> IVGGTASVRGEWPWQVTLHTTSPTQRHLCGGSIIGNQWILTAAHCFYGVESPKILR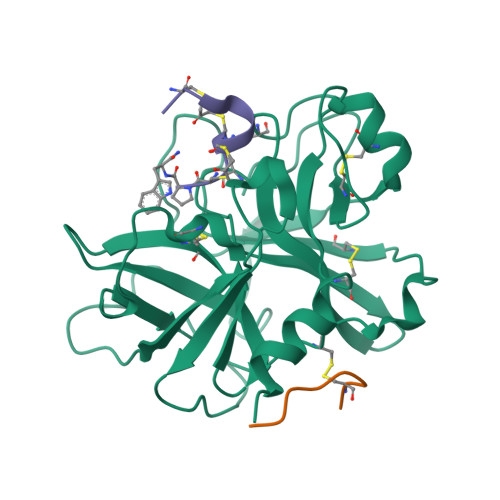VYSGILNQSEIKEDTSFFGVQEIIIHDQYKMAESGYDIALLKLETTVGYGDSQRPICLPSKGDRNVIYTDCWVTGWGYRKLRDKIQNTLQKAKIPLVTNEECQKRYRGHKITHKMICAGYREGGKDACKGDSGGPLSCKHNEVWHLVGITSWGEGCAQRERPGVYTNVVEYVDWILEKTQAVHHHHHH;> TCVNIMCCRCPX;> MDDDDKMDNECTTKIKPR> TLSSQDKPFNLRSRDPIYSNNYGKLYEITPEKNSQLRD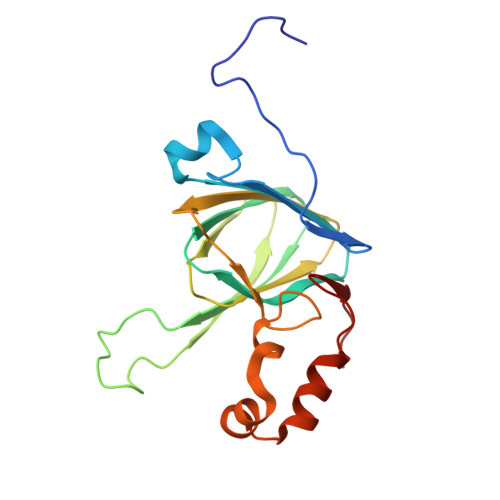LDILLNCLQMNEGALFVPHYNSRATVILVANEGRAEVELVGLEQQQQQGLESMQLRRYAATLSEGDIIVIPSSFPVALKAASDLNMVGIGVNAENNERNFLAGHKENVIRQIPRQVSDLTFPGSGEEVEELLENQKESYFVDGQPR ethyl (2~{S})-2-[(2-chloranyl-6-methyl-phenyl)-thiophen-2-ylcarbonyl-amino]propanoate | C17 H18 Cl N O3 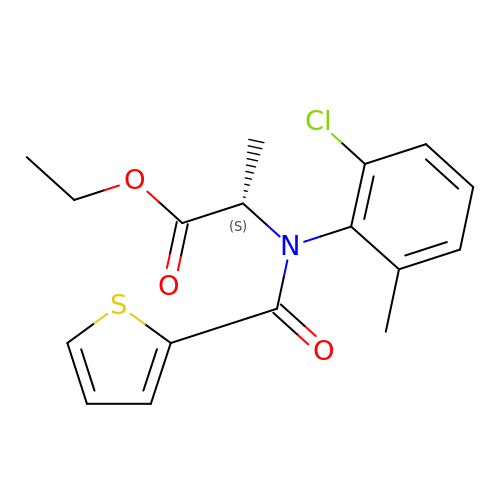S | XYAGVCFCNDDPMS-LBPRGKRZSA-N> SVALVPHVGMGLE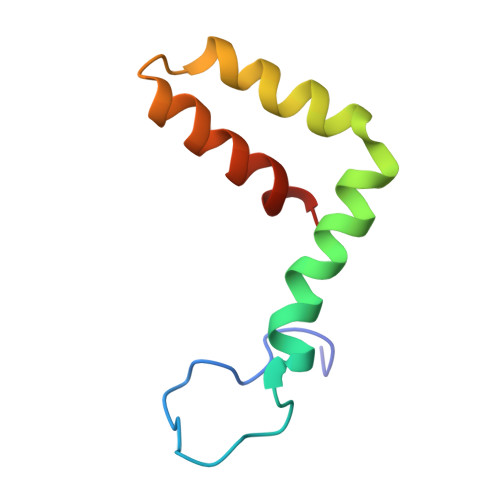TATETWMSSEGAWKHAQRIETWILRHPGFTIMAAILAYTIGTTHFQRALIFILLTAVAPSMT>IASKSMKIGIIGAMEEEVTLLRDKIENRQTITIGGSEIYTGQLHGVDVALLKSGIGKVAAAMGATLLLERCQPDVIINTGSAGGLASTLKVGDIVVSDEARYHDADVTAFGYEYGQLPGCPAGFKADEKLVAAAESCIKALDLNAVRGLIVSGDAFINGSVGLAKIRHNFPQAIAVEMEATAIAHVCHNFKVPFVVVRAISDVADQQSHLSFEEFLAVAARQSTLMVENLVQNLAR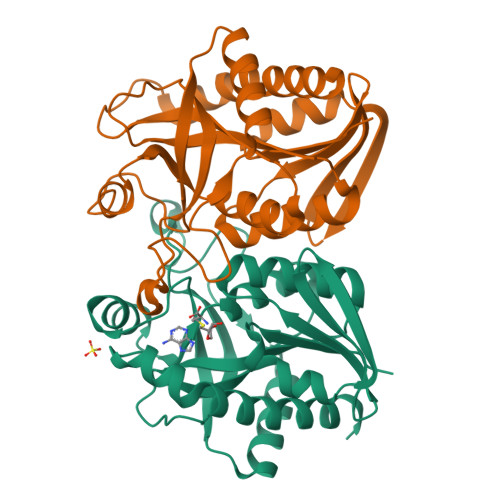G[2x]> XLWQFNGMIKCKIPSSEPLLDFNNYGCYCGLGGSGTPVDDLDRCCQTHDNCYKQAKKLDSCKVLVDNPYTNNYSYSC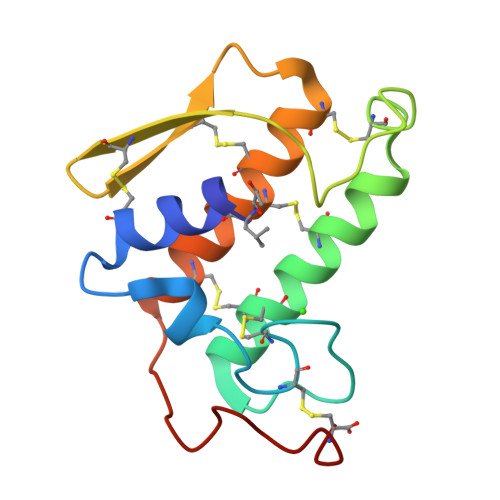SNNEITCSSENNACEAFICNCDRNAAICFSKVPYNKEHKNLDKKNC>MEKRIKGSCTSILVGKKASIDGSTLISRNDPGHEALDPQRFVVVNPEDQPRDYTSVISKVNVKLPDDPQRYTSIPNSILTNGIWPAAGINSSNVAMSATETITTNSRVQGLDPFVENGLGEEDLVTVVLPYVKSAREGVKRLGSLLEEYGTYEPNGISFADNEEVWWLETIGGHHWAAVRIPDDAYVVAPNRMNIDQFDFDSDDT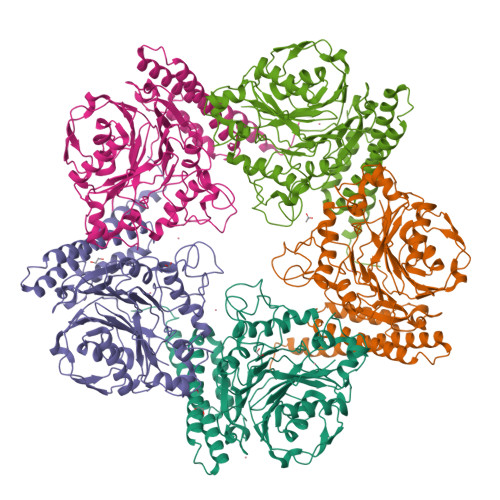LCSSDLKDLIDNNNLNPDFENYNLRHIFGSASIKDTVYNNPRTWYGQKFFSPDDTADDPMEQDLPFICHANRKISVEDVKFVLSSHFENTKYDVYGSGSQSDKTLFRPIGINRNHNVHILQIRNNVPTEIAGIHWLAYGANTFNTVVPFYANVNDTPVQYKNATGKFDLNNMYWLSCTTALLGDTDYDFYVDMRNDYELDAMSAYRKIQNDTDADISGQKDIEKYLENANKKLADVAFEKQNKLLGDMVTTGSNNMKLRYNLND[5x]> AKLGIHSNDTRDAWVNKIAQLNTLEKAAEMLKQFRMDHTTPFRNSYELDNDYLWIEAKLEEKVAVLKARAFNEVDFRHKTAFGEDAKSVLDGTVAKMNAAKDKWEAEKIHIGFRQAYKPPIMPVNYFLDGERQLGTRLMELRNLNYYDTPLEEL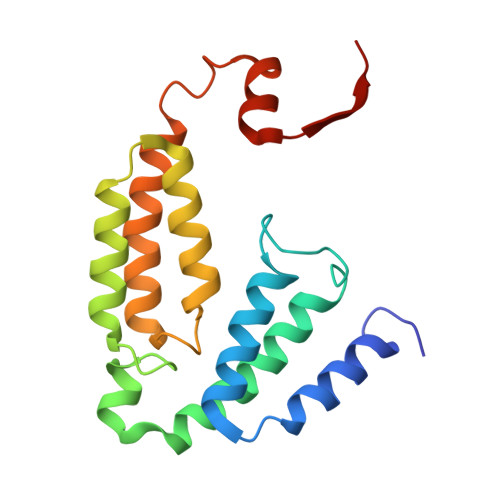RKQRGVRVVHLQSPH>[4x]GTVNNELGYQLFRDFAENKGMFRPGATNIAIYNKQGEFVGTLDKAAMPDFSAVDSEIGVATLINPQYIASVKHNGGYTNVSFGDGENRYNIVDRNNAPSLDFHAPRLDKLVTEVAPTAVTAQGAVAGAYLDKERYPVFYRLGSGTQYIKDSNGQLTKMGGAYSWLTGGTVGSLSSYQNGEMISTSSGLVFDYKLNGAMPIYGEAGDSGSPLFAFDTVQNKWVLVGVLTAGNGAGGRGNNWAVIPLDFIGQKFNEDNDAPVTFRTSEGGALEWSFNSSTGAGALTQGTTTYAMHGQQGNDLNAGKNLIFQGQNGQINLKDSVSQGAGSLTFRDNYTVTTSNGSTWTGAGIVVDNGVSVNWQVNGVKGDNLHKIGEGTLTVQGTGINEGGLKVGDGKVVLNQQADNK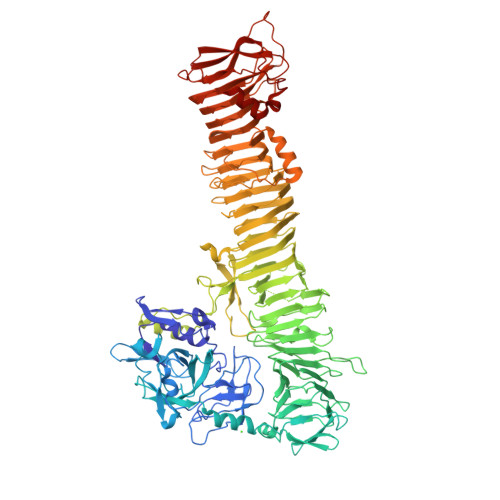GQVQAFSSVNIASGRPTVVLTDERQVNPDTVSWGYRGGTLDVNGNSLTFHQLKAADYGAVLANNVDKRATITLDYAGNTAGYLFHGQLKGNLNVDNRLPEGVTGALVMDGAADISGTFTQENGRLTLQGHPVIHAYNTQSVADKLAASGDHSVLTQPTSFSQEDWENRSFTFDRLSLKNTDFGLGRNATLNTTIQADNSSVTLGDSRVFIDKNDGQGTAFTLEEGTSVATKDADKSVFNGTVNLDNQSVLNINDIFNGGIQANNSTVNISSDSAVLGNSTLTSTALNLNKGANALASQSFVSDGPVNISDATLSLNSRPDEVSHTLLPVYDYAGSWNLKGDDARLNVGPYSMLSGNINVQDKGTVTLGGEGELSPDLTLQNQMLYSLFNGYRNIWSGSLNAPDATVSMTDTQWSMNGNSTAGNMKLNRTIVGFNGGTSPFTTLTTDNLDAVQSAFVMRTDLNKADKLVINKSATGHDNSIWVNFLKKPSNKDTLDIPLVSAPEATADNLFRASTRVVGFSDVTPILSVRKEDGKKEWVLDGYQVARNDGQGKAAATFMHISYNNFITEVN> MGHHHHHHPSGVKTENNDHINLKVAGQDGSVVQFKIKRHTPLSKLMKAYCERQGLSMRQIRFRFDGQPINETDTPAQLEMEDEDTIDVFQQQTGGCMDPPSDAESPVTDDGFTLQLSQDASLCPSNSGTFSIIDVASDRRLFNTFIKEWKTKERYSLALACEKREHIQQPEGEIGGKHKRAPAARQKLNRTDGFPVRDSDGLVLIGLSVCWGARDSYYISLQQEQSKGLSSSLAPPPLDDDLPVSERLGQVRSCLSRPSAGLRGGVVVTYDIIQVYKTLVLSCGISLAGNCEDPKVACWLLDPGSEERTLPNMVTVYCPEELPLLDGLGSAHAHCPRVRAATKSVLVHAVMNHLTGLLEKDSMLDLFRSIEMPSQVCLALLELNGVGFSVEECERQKHVMQAKLTALESQAYNLAGHSFSLTSIDDIAQVLFLELHLPPNGDVGGSKSKKTLGYTRRGGGRVRLGKQFSTTKDILEKLRPLHPLPGVILEWRRITNALTKVVFPLQREKQYHPTLAMDRIYPIAQTHTATGRVSFTEPNIQNVPKDFEICMPTVVGESPPSQNGCQMTTKPGKNRRSVAPSVTGGAAEQGPAFSVSMRHAFVPFSGGMILAADYSQLELRVLAHLSKDQRLLQVLNGGADVFRCIAAEWKGVDPETVNDSLRQQAKQICYGIIYGMGAKSLGEQMGVEENDAACYIESFKARYKGINAFLKETVKNCIKNGYVQTLMGRRRYLPGISNTNTHIKAHAERQAVNTTVQGSAADIVKLATVNIQKRLRKTYPTAPLSHQHTHSGTSQYRAGTSHLRGAFFVLQLHDELIYETREEDLIQVAQIVKREMESAVKLYVKLKAKVKVGPSWGNLQDLDL

DNA polymerase θ (Pol θ) plays an essential role in the microhomology-mediated end joining (MMEJ) pathway for repairing DNA double-strand breaks. Pol θ catalyzes the annealing of microhomologous DNA ends and performs template-dependent DNA extension. Distinct from its homologs in DNA replication, Pol θ-pol exhibits low fidelity and possesses TLS activities. In this work, we characterized a Pol θ-pol homolog from vertebrate Lates calcarifer (Lc), which shares high sequence and functional similarities with HsPol θ-pol.

To assemble the ternary complex, LcPol θ-pol was incubated with the incoming nucleotide dGTP, Mg2+, and a DNA duplex (20/29 mer) with a dideoxy-A (ddA)-terminating end, to prevent chain elongation. Final 3D reconstruction and refinement yielded two structures at 2.4 Å (complex Ia) and 2.8 Å (complex Ib). 11 and 18 bp of the duplex DNA are visible in complexes Ia and Ib, respectively. In complex Ia, the DNA substrate around the minor groove contacts the thumb domain. R2342, K2322 and R2343 interact with the primer backbone, and T2272 and D2275 are in proximity to the template backbone. The finger domain in both complexes Ia and Ib exists in a closed state with the incoming dGTP and one Mg2+ ion bound to the active site. The 2.4 Å structure of the LcPol θ-pol complex Ia allows confident modeling of the active site. The B-site Mg2+ is coordinated by three oxygen atoms on the incoming dGTP, D2463, D2664, and the backbone of Y2464. The finger domain movement brings R2512, K2516 and Y2520 to contact the triphosphate group of dGTP. The nascent base pair is surrounded by a series of hydrophilic residues, with Q2534, Q2517, and K2516 on one side, and R2382, Q2607 and N2603 on the other side.>DPTQFEERHLKFLQQLGKGNFGSVEMCRYDPLQDNTGEVVAVKKLQHSTEEHLRDFEREIEILKSLQHDNIVKYKGVCYSAGRRNLKLIMEYLPYGSLRDYLQKHKERIDHIKLLQYTSQICKGMEYLGTKRYIHRDLATRNILVENENRVKIGDFGLTKVLPQDKEYY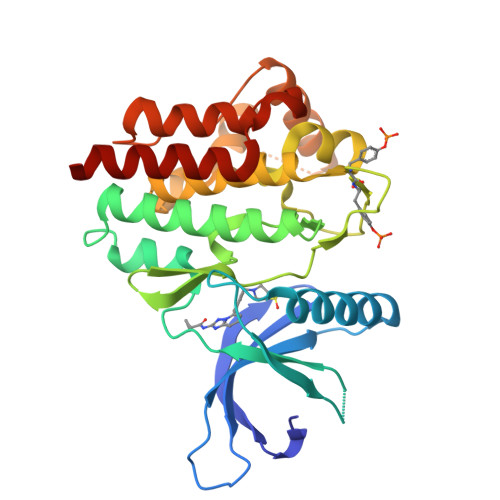KVKEPGESPIFWYAPESLTESKFSVASDVWSFGVVLYELFTYIEKSKSPPAEFMRMIGNDKQGQMIVFHLIELLKNNGRLPRPDGCPDEIYMIMTECWNNNVNQRPSFRDLALRVDQIRDQMAG[2x]> GAASMSPSASDNSCAYCGIDSAKCVIKCNSCKKWFCNTKNGTSSSHIVNHLVLSHHNVVSLHPDSDLGDTVLECYNCGRKNVFLLGFVSAKSEAVVVLLCRIPCAQTKNANWDTDQWQPLIEDRQLLSWVAEQPTEEEKLKARLITPSQISKLEAKWRSNKDATINDIDAPEEQEAIPPLLLRYQDAYEYQRSYGPLIKLEADYDKQLKESQALEHISVSWSLALNNRHLASFTLSTFESNELKVAIGDEMILWYSGMQHPDWEGRGYIVRLPNSFQDTFTLELKPSKTPPPTHLTTGFTAEFIWKGTSYDRMQDALKKFAIDKKSISGYLYYKILGHQVVDISFDVPLPKEFSIPNFAQLNSSQSNAVSHVLQRPLSLIQGPPGTGKTVTSATIVYHLSKIHKDRILVCAPSNVAVDHLAAKLRDLGLKVVRLTAKSREDVESSVSNLALHNLVGRGAKGEL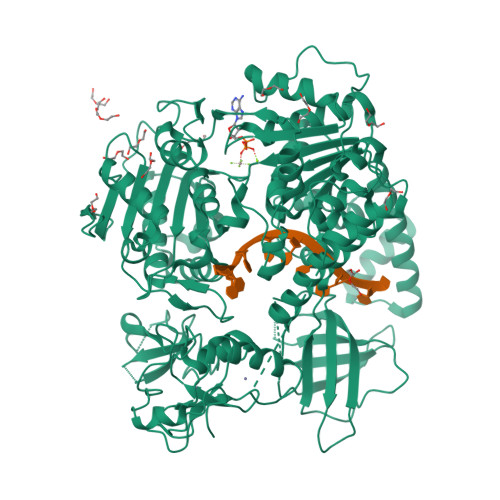KNLLKLKDEVGELSASDTKRFVKLVRKTEAEILNKADVVCCTCVGAGDKRLDTKFRTVLIDESTQASEPECLIPIVKGAKQVILVGDHQQLGPVILERKAADAGLKQSLFERLISLGHVPIRLEVQYRMNPYLSEFPSNMFYEGSLQNGVTIEQRTVPNSKFPWPIRGIPMMFWANYGREEISANGTSFLNRIEAMNCERIITKLFRDGVKPEQIGVITPYEGQRAYILQYMQMNGSLDKDLYIKVEVASVDAFQGREKDYIILSCVRANEQQAIGFLRDPRRLNVGLTRAKYGLVILGNPRSLARNTLWNHLLIHFREKGCLVEGTLDNLQLCTVQLV> SGRENLYFQGHMKPQVYHVDAFTSQPFRGNSAGVVFPADNLSEAQMQLIARELGHSETAFLLHSDDSDVRIRYFTPTVEVPICGHATVAAHYVRAKVLGLGNCTIWQTSLAGKHRVTIEKHNDDYRISLEQGTPGFEPPLEGETRAAIINALHLTEDDILPGLPIQVATTGHSKVMIPLKPEVDIDALSPDLNALTAISKKIGCNGFFPFQIRPGKNETDGRMFSPA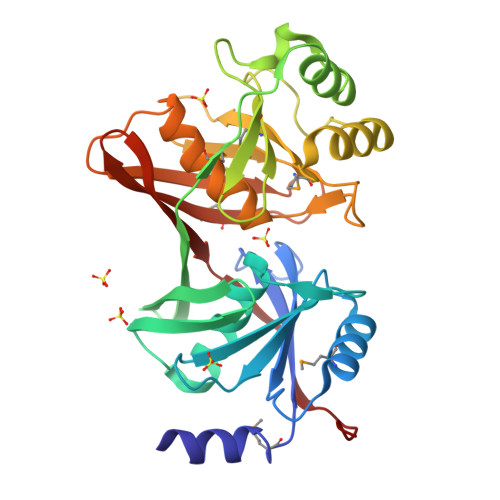IGIVEDPVTGNANGPMGAWLVHHNVLPHDGNVLRVKGHQGRALGRDGMIEVTVTIRDNQPEKVTISGTAVILFHAEWAIELGS>MIMIMASKSSPHDLPDVSGLSIAVLGGTGDQGRGLARRFAMAGHEVILGSRSAERAQAVAAELGEGLPVRGMDNAGAAEAGDVVIVAVPWDGHRALLESLKDVLAGKIVVDCVNPLGFDKRGAYALPVEEGSAAEQAAAILPDSRVVAAFHHVSAVLLLDPEVEKVDLDVLVLGDDREATDVVRALAARIPGVRGVYGGRLRNAHQVE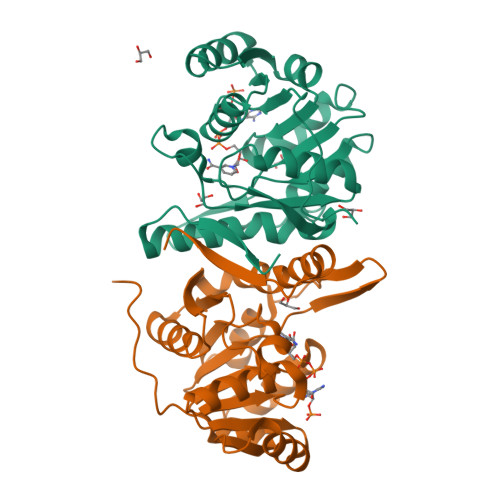AFTANLISINRRYKAHAGIRITDI[4x]>[2x]MKETTIFAMHLGKALDPNLPVFVKAEKDTNIKLVNVASQNQTDQIQAYNLMLTEGKLPDIVSYELSADLENLGIEGGLIPLEDLINQHAPNLKKFFEENPRYKKDAVAVDGHIYMIPNYYDYFNIKVSQGYFIRQDWLEKLGLKEPRTVDELYTTLKAFREKDPNGNGKKDEVPFFVRANNVRKVLTSLVDLFKASPIWYEENGMVKYGPAQKEFKHAIKELSKWYKEGLIDEEIFTRGLESRDYLLSNNLGGATDDWIASTSSYNRNLADKIPGFNLKLVLPYELNGNAKTRHARTTYLGGWGISKDAKDPVSLIKYFDYWYSVEGRRLWNFGIEGSEYTLVDGKPVFTDKVLKNPDGKTPLAVLREVGAQYRLGAFQDAQYELGWASESAKAGYKYYMDNDVVLDELPILKYTKEKSKEFVSIDTAMRAVVEEKAQQWILGSGDIDKEWDAYIKRLENLGLSKAEQIQNEAF

A periplasmic solute-binding protein (Smon0123) captures unsaturated GAG disaccharides with the 1,3-glycoside bond and delivers substrates to an ABC transporter localized in the cytoplasmic membrane. Smon0123 is composed of two major domains (N- and C-domains), and each domain has two small subdomains. Each domain included a parallel and an antiparallel β-sheet surrounded by many α-helices and formed the α/β sandwich structure. All the crystal structures of Smon0123 so far determined include metal ion in its molecule, suggesting that the metal ion contributes to protein folding.

Crystal structures of ligand-free Smon0123 (N-28/C-5) and ligand (CΔ4S or CΔ6S)-bound Smon0123 (N-18/C-5) were also determined by molecular replacement with CΔ0S-bound Smon0123 (N-18/C-5). Generally, the solute-binding protein adopts two conformations during substrate binding, substrate-free open form and substrate-bound closed form, indicating that there is a transitional state (substrate-bound open form) in the conformational change. Compared with the structure of CΔ0S-bound Smon0123 and that of ligand-free Smon0123, the N- and C-domains of ligand-bound Smon0123 were 47° more closed than those of ligand-free Smon0123. Distinct from substrate-free Smon0123 in the open conformation, the binding protein in complex with the substrate adopts the closed conformation by accommodating the substrate at the cleft between the N- and C-domains. Therefore, the closed conformation of substrate-bound Smon0123 is considered to be important for association with the ABC transporter. The substrate specificity of Smon0123 coincided with that of Smon0121-Smon0122(10xHis)/Smon0120-Smon0120 for ATPase activity, indicating that the ABC transporter interacts with substrate-bound Smon0123 (closed form), but not the substrate-free form, and triggers ATP hydrolysis.> TEQQWNFAGIEAAASAIQGNVTSIHSLLDEGKQSLTKLAAAWGGSGSEAYQ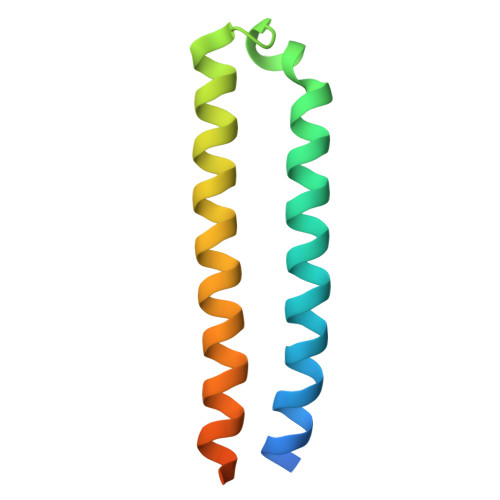GVQQKWDATATELNNALQNLARTISEAGQAMASTEGNVTGMFA> EQARPADDALAALGAQLFVDPALSRNATQSCATCHDPARAFTDPREGKAGLAVSVGDDGQSHGDRNTPTLGYAALVPAFHRDANGKYKGGQFWDGRADDLKQQA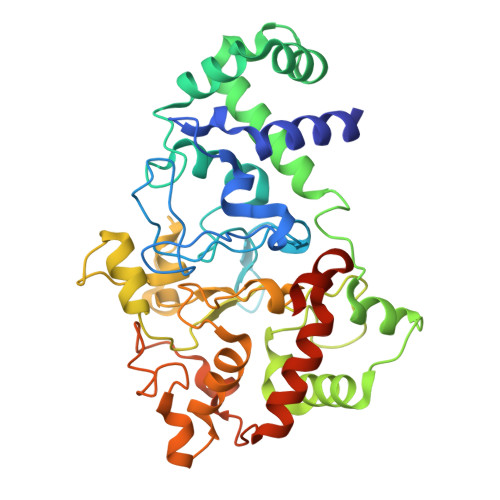GQPMLNPVEMAMPDRAAVAARLRDDPAYRTGFEALFGKGVLDDPERAFDAAAEALAAYQATGEFSPFDSKYDRVMRGEEKFTPLEEFGYTVFITKNCRLCHMQRKQGVAERETFTNFEYHNIGLPVNETAREASGLGADHVDHGLLARPGIEDPAQSGRFKVPSLRNVAVTGPYMHNGVFTDLRTAILFYNKYTSRRPEAKINPETGAPWGEPEVARNLSLAELQSGLMLDDGRVDALVAFLETLTDRRYEPLLEESRAAQKDHHHHHH>[4x]MAAGVAAWLPFARAAAIGWMPVASGPMPAPPRQERKRTQDALIVLNVSGTRFQTWQDTLERYPDTLLGSSERDFFYHPETQQYFFDRDPDIFRHILNFYRTGKLHYPRHECISAYDEELAFFGLIPEIIGDCCYEEYKDRRRENAERLQDDADTDTAGESALPTMTARQRVWRAFENPHTSTMALVFYYVTGFFIAVSVIANVVETVPCGSSPGHIKELPCGERYAVAFFCLDTACVMIFTVEYLLRLAAAPSRYRFVRSVMSIIDVVAILPYYIGLVMTDNEDVSGAFVTLRVFRVFRIFKFSRHSQGLRILGYTLKSCASELGFLLFSLTMAIIIFATVMFYAEKGSSASKFTSIPAAFWYTIVTMTTLGYGDMVPKTIAGKIFGSICSLSGVLVIALPVPVIVSNFSRIYHQNQRADKRRAQKKARLARIRAAKSGSANAYMQSKRNGLLSNQLQSSEDEQAFVSKSGSSFETQHH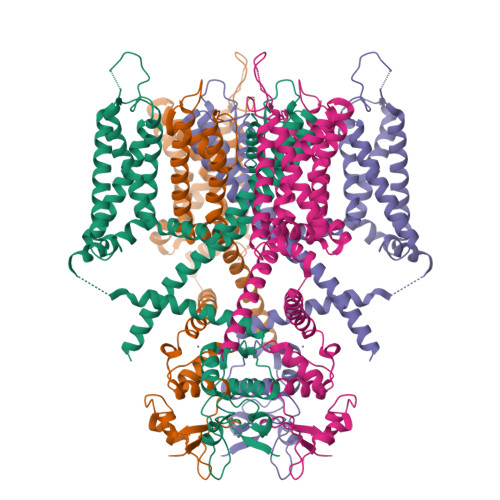HLLHCLEKTTNHEFVDEQVFEESCMEVATVNRPSSHSPSLSSQQGVTSTCCSRRHKKTFRIPNANVSGSHQGSIQELSTIQIRCVERTPLSNSRSSLNAKMEECVKLNCEQPYVTTAIISIPTPPVTTPEGDDRPESPEYSGGNIVRVSAL>MSVVGTPKSAEQIQQEWDTNPRWKDVTRTYSAEDVVALQGSVVEEHTLARRGAEVLWEQLHDLEWVNALGALTGNMAVQQVRAGLKAIYLSGWQVAGDANLSGHTYPDQSLYPANSVPQVVRRINNALQRADQIAKIEGDTSVENWLAPIVADGEAGFGGALNVYELQKALIAAGVAGSHWEDQLASEKKCGHLGGKVLIPTQQHIRTLTSARLAADVADVP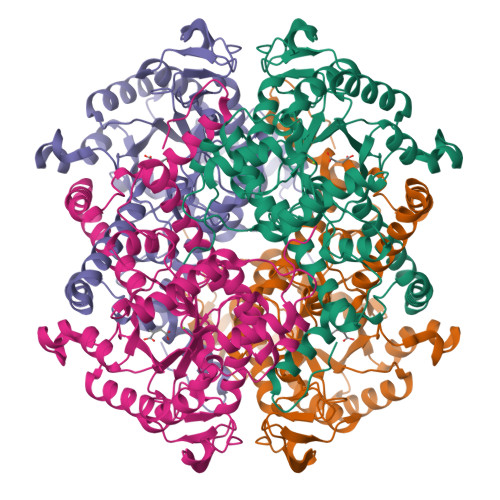TVVIARTDAEAATLITSDVDERDQPFITGERTREGFYRTKNGIEPCIARAKAYAPFADLIWMETGTPDLEAARQFSEAVKAEYPDQMLAYNCSPSFNWKKHLDDATIAKFQKELAAMGFKFQFITLAGFHALNYSMFDLAYGYAQNQMSAYVELQEREFAAEERGYTATKHQREVGAGYFDRIATTVDPNSSTTALTGSTEEGQFHLEHHHHHH[2x]>[6x]MKHHHHHHHHGGLVPRGSHGGSEFMTVDEQVSNYYDMLLKRNAGEPEFHQAVAEVLESLKIVLEKDPHYADYGLIQRLCEPERQLIFRVPWVDDQGQVHVNRGFRVQFNSALGPYKGGLRFHPSVNLGIVKFLGFEQIFKNSLTGLPIGGGKGGSDFDPKGKSDLEIMRFCQSFMTELHRHIGEYRDVPAGDIGVGGREIGYLFGHYRRMANQHESGVLTGKGLTWGG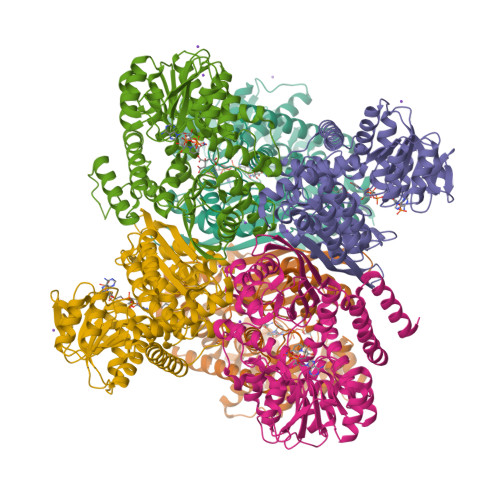SLVRTEATGYGCVYFVSEMIKAKGESISGQKIIVSGSGNVATYAIEKAQELGATVIGFSDSSGWVHTPNGVDVAKLREIKEVRRARVSVYADEIEGATYHTDGSIWDLKCDIALPCATQNELNGENAKTLADNGCRFVAEGANMPSTPEAVEVFRERDIRFGPGKAANAGGVATSALEMQQNASRDSWSFEYTDERLQVIMKNIFKTCAETAAEYGHENDYVVGANIAGFKKVADAMLAQGVI>[2x]MFENITAAPADPILGLADLFRADERPGKINLGIGVYKDETGKTPVLTSVKKAEQYLLENETTKNYLGIDGIPEFGRCTQELLFG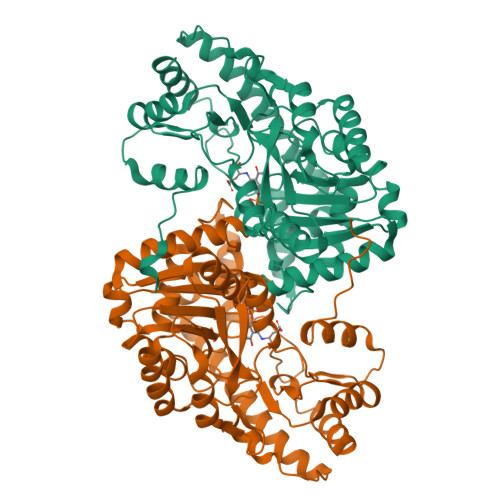KGSALINDKRARTAQTPGGTGALRVAADFLAKNTSVKRVWVSNPSWPNHKSVFNSAGLEVREYAYYDAENHTLDFDALINSLNEAQAGDVVLFHGCCHNPTGIDPTLEQWQTLAQLSVEKGWLPLFDFAYQGFARGLEEDAEGLRAFAAMHKELIVASSYSKNFGLYNERVGACTLVAADSETVDRAFSQMKAAIRANYSNPPAHGASVVATILSNDALRAIWEQELTDMRQRIQRMRQLFVNTLQEKGANRDFSFIIKQNGMFSFSGLTKEQVLRLREEFGVYAVASGRVNVAGMTPDNMAPLCEAIVAVL> KWIYKFDVLYQSRNPRYRNYEIIRTNVQEVLAEIVSPSTKNPNSENPAVKKRFRGIKNVVSRIISNDKKCRYDLIYNKYLSSSDTRKLKTMIDYSTKFNRVVEVVLIIMGKLLPLDAWGGTENKKVIQDRIVDFLRLGANERLHLDDVLSGIKLSKFKWLGVGNNISSQQDFQIRKRLLEGYINWVFISLVKNIVRAFWYVTESSNMDRSKLFYFTHSIWNELSSNWITKYAKGNLVQVVSPESKGQFTNGKIKLIPKRGGFRVICVPLKQSLYSFNNKRNFALKQKEKWDYIFYQKYTLSPVRQVLQLKLNALRKSDMGHRSSVNSTNEVADRILTFRNDLLKKNKTLPVLYMIKFDMKECYDRLNQNALKESIAGIFKEDNENTTYHVREYGTLDEFLKLKRVRTLIETEVQNFNIIMNSKDEAEAGSRSYGTKVDKVKTLSISKNKIIEVCHSQIEDATCLVKNKEGQYDLFKRKQGVFQGFSLSGIFCDILYSTMVSKEFKFLWEATEDNLLLRLVDDFIFITSNKDTLKKVKDKISSNELQKYGAFVNHEKTVEINGEAGSSNKMTFVGLDINCLTLDVKKDSSQF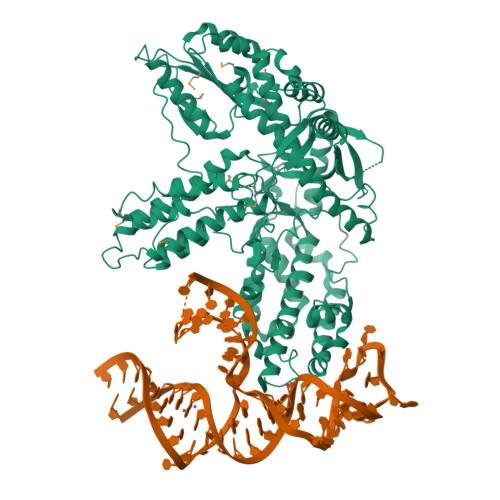SRPTCKFRSFKALFSNLKQFYCSNLSEFLLDFSSNSLETIRENVDAILKLTFEAIQTSFATISKQDSFERYRFMKFLHVIIETTIEKFARVNGSMEGVEYLLTCIKITITKSLAFMATKQEIIEWLYTLTIVD>[2x]GIDPFTARPSSSMADFRKFFAKAKHIVIISGAGVSAESGVPTFRGAGGYWRKWQAQDLATPLAFAHNPSRVWEFYHYRREVMGSKEPNAGHRAIAECETRLGKQGRRVVVITQNIDELHRKAGTKNLLEIHGSLFKTRCTSCGVVAENYKSPICP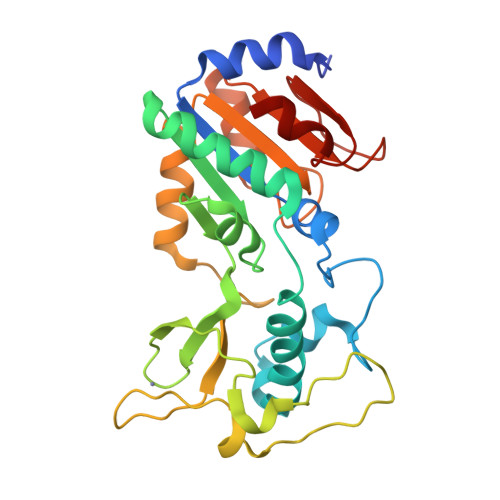ALSGKGAPEPGTQDASIPVEKLPRCEEAGCGGLLRPHVVWFGENLDPAILEEVDRELAHCDLCLVVGTSSVVYPAAMFAPQVAARGVPVAEFNTETTPATNRFRFHFQGPCGTTLPEALA> MARHFVLNTGAKIPSVGLGSWQSDPGVVGNAVYAAVKAGYRHIDCARVYGNEKEIGLALKKLFEEGVVKREDMFITSKLWNDHHAPEDVPEALNDSLNDLQLEYLDLYLIHWPFRVKKGTNTSPENFVTPDF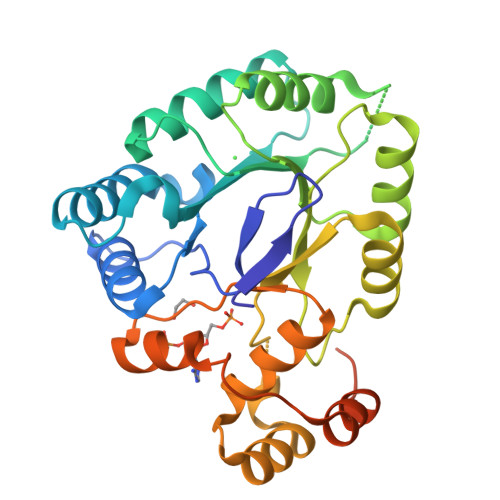PATWGAMEKLYDAGKARAIGVSNFSSKKLGDLLAVARVPPAVDQVECHPGWQQTKLHSFCQSTGVHLTAYSPLGSPGTTWMNGNVLKEPIIISIAEKLGKTSAQVALRWNIQMGHSVLPKSTNEERIKQNLDVYDWSIPDDLLAKFSEIKQARLLRGNFIVNPESVYKTHEELWDGEL1,3-DIPHENYL-1H-PYRAZOLE-4,5-DICARBOXYLIC ACID 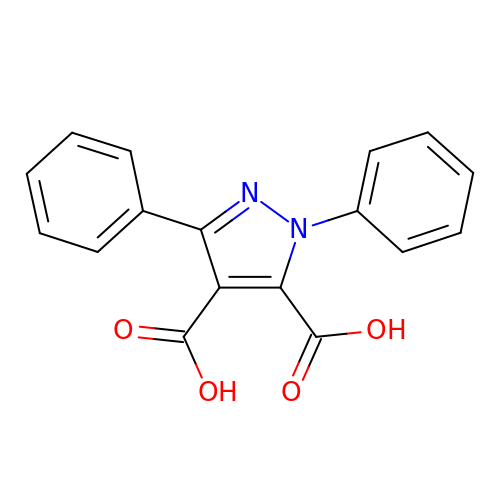| C17 H12 N2 O4 | WERNQSNSNVDBBJ-UHFFFAOYSA-N> SNARNKIFISHAAPDDNDFTKWLALKLIALGYEVWCDVLFLDKGADFWKVIDKEIREGAIKFLLATSEIAIKRDGVLKEIAVAEKVKKQLKDDNFIIPLIIDENLSYDDLPPEIIRLNAVDFKKSWAVGLQDLLKALDDQKVEKNSPDPDKSNALYQQIFLHNKGIIEREEIYDSNWFSILSFPKELRFHDYEKLMPKGFDVRELTYPAVRYKNYLCTFAWEYDFMHQLPKTETYNSSQTIRIPTEEILSGKYDSPFIGNFECQRLIVQLLNKAFELRMKEKGVREYPMSNKMGYWFEKGKL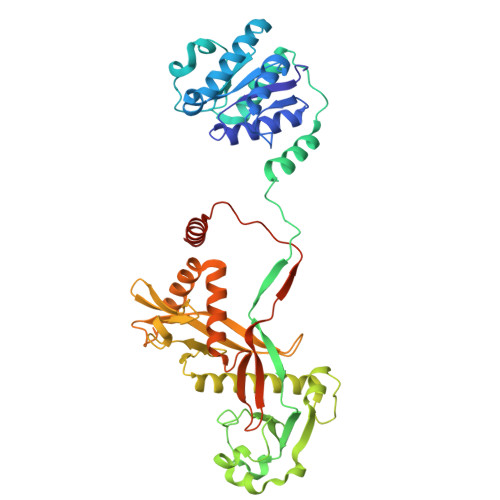EKDKFNKVLLVGKQKDKHWHFGISAAGKLYPFPVLMISSHIFFTKDGKELIESKKIQHAARRRQGKNWWNDDWRNKLLAFVKYLSDDENSFYLEVGSEEKIYISNEPVQFVGKVSYNMPEKNNLKDEAEISDLNDLNEFDGEIFEETDSE> MNGWNFQELKETPSQTGGPYVHIGLLPKQANIEVFEHNLDNNLVQDNTQGQRIRLEGQVFDGLGLPLRDVLIEIWQADTNGVYPSQADTQGKQVDPNFLGWGRTGADFGTGFWSFNTIKPGAVPGRKGSTQAPHISLIIFARGINIGLHTRVYFDDEAEANAKDPVLNSIEWATRR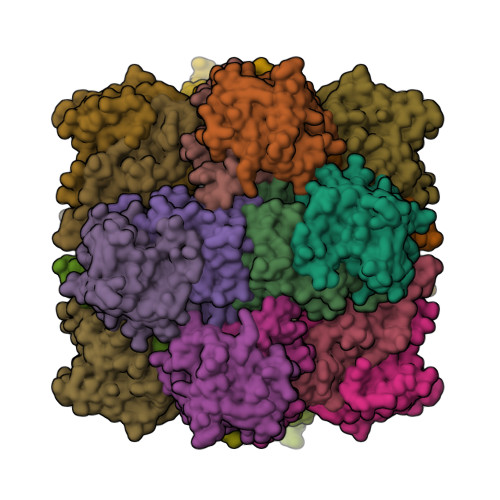QTLVAKREERDGEVVYRFDIRIQGENETVFFDI;> MSQIIWGAYAQRNTEDHPPAYAPGYKTSVLRSPKNALISIAETLSEVTAPHFSADKFGPKDNDLILNYAKDGLPIGERVIVHGYVRDQFGRPVKNALVEVWQANASGRYRHPNDQYIGAMDPNFGGCGRMLTDDNGYYVFRTIKPGPYPWRNRINEWSPAHIHFSLIADGWAQRLISQFYFEGDTLIDSCPILKTIPSEQQRRALIALEDKSNFIEADSRCYRFDITLRGRRATYFENDLT>MKGYTVPLSPRGIANLAPAPPWHYAGTVVGVEFFTDPAAAAATLPEGLTPDPDSAGRGVAMFIDWQYSSTGLEYLDPARSQYREFLITLDAHCNGAPVAWCPYIYVDNDAAMARGWVQGFPKKLGAVHQTRAYSVGGPGTPVLGPGGQFGAT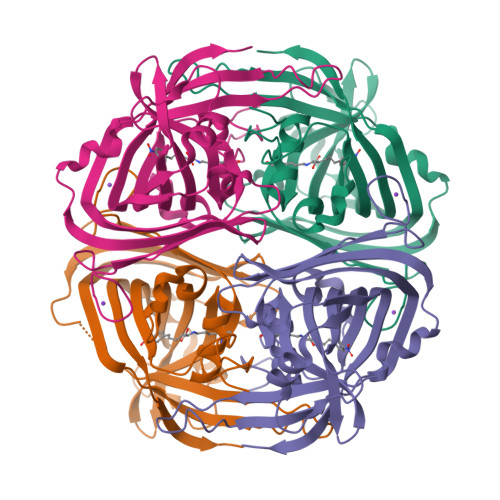ASSAGQRIAEAKITLEQPVPDPAALMSRPVINLRHFPRLAAGQHDQPAVHELVMSVLDDTAVSDAWVGTADLAFLPAHGEELADLPVRRTGKGFHFDLAFTVTDLMTLADHSA[4x]>WSHPQFEKENLYFQSMANVIKARPKLYVMDNGRMRMDKNWMIAMHNPATIHNPNAQTEFVEFPIYTVLIDHPEGKILFDTSCNPNSMGPQGRWAESTQQMFPWTATEECYLHNRLEQLKVRPEDIRYVVASHLHLDHAGCLEMFTNATIIVHEDEFNGALQCYARNQKEGAYIWADIDAWIKNNLQWRTVKRHEDNILLAEGVKVLNFGSGHAWGMLGLHVELPETGGIILASDAIYTAESYGPPIKPPGIIYDSLGYMNTVERIRRIAQETKSQVWFGHDAEQFKKFRKSTEGYYE[3x]

MLLs degrade N-acyl-L-homoserine lactones (AHLs), molecules that are used in a microbial communication system called quorum sensing (QS) to coordinate a variety of behaviors, including virulence and biofilm formation. We provide the structural and biochemical analysis of the lactonase GcL (WP_017434252.1), isolated from the thermophilic bacteria Parageobacillus caldoxylosilyticus. GcL is a thermostable, highly proficient lactonase with broad substrate specificity (kcat/KM values range between 104 to 106 M–1 s–1) for substrates such as N-butyryl (C4) L-homoserine lactone (HSL) and N-decanoyl (C10)-HSL. The binuclear center, common to all MLLs, is coordinated by five histidine residues and two aspartic acid residues.

We solved the structure of GcL in complex with AHL-hydrolytic products bound to the active site through cocrystallization with C8-HSL. While the model of GcL in complex with the hydrolytic product of C8-HSL is limited in its accuracy by a relatively low ligand occupancy (∼0.7), it reveals that the negative charge of the hydrolytic product carboxylate group is stabilized by the bimetallic active site center, and that the alcohol group interacts with the α-metal (iron; 2.7 Å; monomer L). In addition, the carboxylate group of the C8-HSL product is positioned between the two metal cations, 2 Å from the cobalt cation and 2.8 Å from the iron cation (monomer L). The other oxygen atom of the carboxylate is hydrogen bonded to the hydroxyl group of Tyr223 (2.7 Å). During lactone hydrolysis, the protonation of the leaving alcoholate group may be an important, catalytically limiting step. The position of the alcohol group is 3.3 and 3.5 Å from Asp122 and Tyr223, respectively. This suggests that the side chains of Tyr223 and Asp122 are possible acid catalysts for the reaction, although a protonated Asp122 side chain (protonated in the first reaction step) would be expected to have a more favorable pKa to fulfill the role of an acid catalyst.>[4x]HHHHAYYSMYLKEIFVDNFRNLKKQKLEFCEGVNLIYGLNAQGKSNLLEAIRLLSMGRSFRGSKMSELVKFDEEYFYVRGLVRSADFYEKKIEFGYKVNGNKVIKVNGNKLKSTGEILGHFLTVIFSPEDIEIIKEGPSRRRKYLDACISVIDKNYFFDLLQYNKTLSNRNSLLKKIKEEGKGEDLLEIFDEKLAEYGARI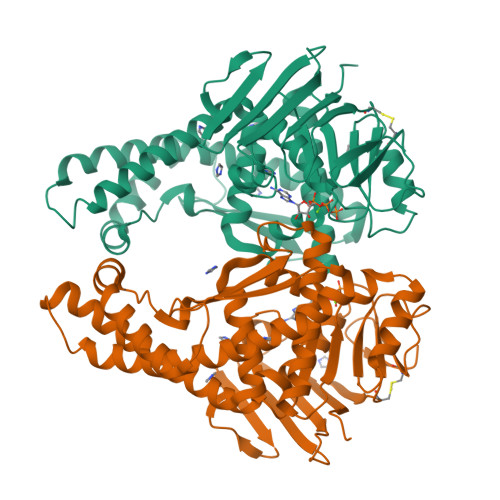IKVRNNYLEKLKNSMSKFLMEISNEKLEIIYLNSAGVKEVHEENLIREKLKNRLTKSLTLDLKYLSTQVGPHREDFKILINGYDSRVYSSQGQKRTAALCLKLSELEILEEETGEKPVLLLDDVMSELDDNRKKYILKKLEGFQSFITHTSKSDVEGDCCFKIYDGIVDKLA> TPPCTQERHYEHLGRCCSRCEPGKYLSSKCTPTSDSVCLPCGPDEYLDTWNEEDKCLLHKV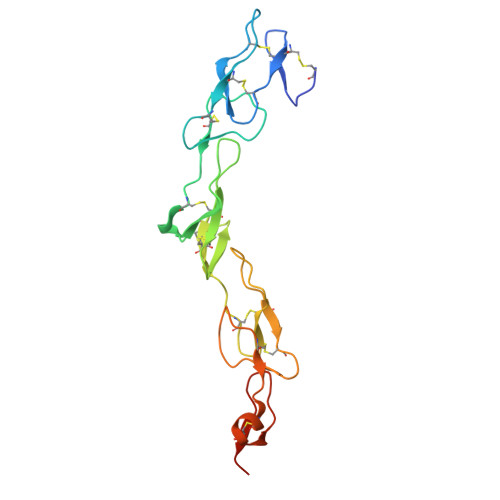CDAGKALVAVDPGNHTAPRRCACTAGYHWNSDCECCRRNTECAPGFGAQHPLQLNKDTVCTPCLLGFFSDVFSSTDKCKPWTNCTLLGKLEAHQGTTESDVVCSSSMTL The essential and metabolic enzyme adenylate kinase (AK) undergoes large-scale conformational changes in response to binding of its substrates ATP and AMP. In addition to the well-characterized ATP- and AMP-binding domains (ATPlid and AMPbd, respectively), the enzyme has three functional loop segments including the p-loop, the selectivity loop, and the catalytic loop. Here, based on a comparative structure–function analysis of AK enzymes from E. coli and the archaea Odinarchaeota and from human AK1, we found that conformational changes in the enzymes are to a varying degree linked to bending, fraying, or unfolding/folding events of the termini of α-helices observed in various structural hot spots of the enzymes.

A notable and distinct feature between the native and Ap5A-bound forms is present in the AMPbd, where the last three residues Ile73, Ser74, and Leu75 in the α-helix spanning residues Arg59–Leu75 change to a flexible conformation when bound to Ap5A. One key interaction site to maintain the helical form of residues Ile73–Leu75 is a network of hydrogen bonds between the side chain of Arg2 and Ser74, as well as to the main chain carbonyl oxygens of Ser74, Thr77, Asp78, and Ile106. To test whether further destabilization of the helical nature of the segment, by itself, can drive closing of the AMPbd and modulate the activity of OdinAK, we substituted Ser74 for a glycine residue. The crystallographic structure of the OdinAK Ser74Gly variant in its substrate-free (apo) form was determined to be 3.6 Å. Despite the relatively low resolution, it is clear that the overall fold of the Ser74Gly variant adopts the expected conformation with the AMPbd in a typical open conformation. In comparison to the native OdinAK structure, there are only minor structural differences near the Ser to Gly substitution. A glycine at position 74 seems to preserve the overall conformation of the S74-helix and does not initiate the unfolding and translational event that is observed in the open-to-closed trajectory in native OdinAK. The catalytic (k cat) activity of the Ser74Gly variant was found to be 0.1 ± 0.003 s–1 at 25 °C which is approximately a 5-fold decrease relative to that of the wild type (k cat = 0.5 ± 0.2 s–1 at 25 °C). Collectively, the results suggest that there is a network of interactions driving the conformational dynamics underlying catalysis in OdinAK and that the loss of one hydrogen bond to Arg2, as well as the destabilizing energetic contribution of an internal glycine (approximately 4 kJ mol–1 ), is not sufficient to drive the conformational change of the S74-helix during subdomain closure. Hence, the local unfolding reaction in OdinAK, although necessary for the closing of the AMPbd, cannot be provoked by the replacement of Ser74 with a helix-breaking glycine residue.

>[6x]MRFILTGVPGAGKTTVCNKLAEKMSNLSVVNYGDVIFEEAKKLYPSIIQVREDTRKLPRADYRNIQIEAAKKIGLITDNLIVDTHMSLKTPYGFYPGLIPETINIIQPDGIILLEFNPRDVIARREKDRLAGKRVTRDMESETDILLHQQVNRMFAVSYSAINQCYVKIIDLTWPQEYEFQHTEYAVNKIIEMLNFKI> MANSTAELEELLMQRSLTDPQLQAAAAAAADFRILPDATVIKIGGQSVIDRGRAAVYPLVDEIVAARKNHKLLIGTGAGTRARHLYSIAAGLGLPAGVLAQLGSSVADQNAAMLGQLLAKHGIPVVGGAGLSAVPLSLAEVNAVVFSGMPPYKLWMRPAAEGVIPPYRTDAGCFLLAEQFGCKQMIFVKDEDGLYTANPKTSKDATFIPRISVDEMKAKGLHDSILEFPVLDLLQSAQHVREVQVVNGLVPGNLTRALAGEHVGT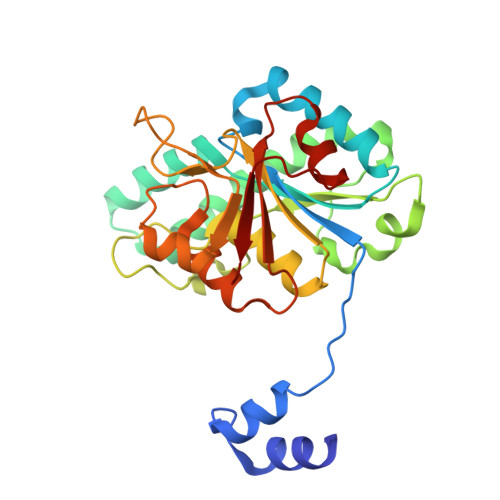IITAS> PSRANTKVIVVGGGGTIGSSTALHLVRSGYTPSNVTVLDAYPIPSSQSAGNDLNKIMDADADPAADAARQMWNEDELFKKFFHNTGRLDCAHGEKDIADLKKRYQNLRDWGLGATVEWLDSEDEILKRMPQLTRDQIKGWKAIFSKDGGWLAAAKAIKAIGEYLRDQGVRFGFYGAGSFKQPLLAEGVCIGVETVDGTRYYADKVVLAAGAWSPTLVELQEQCVSKAWVYGHIQLTPEEAARYKNSPVVYNGDVGFFFEPNEHGIIKVCDEFPGFTRFKMHQPFGAKAPKRISVPRSHAKHPTDTIPDASIVRIRRAIATFMPQFKNKPLFNQAMCWCTDTADGHLLICEHPEWKNFYLATGDSGDSFKLLPIIGKYVVELLEGTLADELAHKWRWRPGSGDALKSRREAPAKDLADMPGWNHD

Fructosyl peptide oxidases (FPOX) are deglycating enzymes that find application as key enzymatic components in diabetes monitoring devices. The inability of wild type FPOXs to act on intact proteins is the most critical issue limiting both their diabetes detection efficiency and their protein deglycation potential. This is due to their buried active site and narrow access tunnel, as determined in multiple crystal structures. In that account, using a rational design approach involving a five-amino acid deletion at the entrance of the active site and a number of further mutations, we described a stable PnFPOX mutant (named L3-35A) that, relative to the wild type enzyme, features a significantly wider and shorter access tunnel.

In the present study, we set out to enhance the thermal stability of the L3-35A mutant by implementing a methodological approach whereby different thermal stabilization strategies are tested in parallel and their efficiency compared. These various strategies involved mutations to either improve the RMSF of the protein (generating mutants hereafter referred to as D-series mutants), increase the number of salt bridges (C-series mutants) or form disulfide bonds (X-series mutants). Our MD-based ranking led to the selection of six candidate mutants (C16, D02, X01, X02A, X04, and X07) for experimental production and characterization. The D02 variant, which relative to L3-35A features two additional mutations (V110R and D115G), shows an increase in Tm of ≈ 1.5 °C with respect to the parent enzyme. We observed that the activity of the enzyme variants towards fK and fV remained similar to that of the parent enzyme, with a slight increase of activity in the case of D02 and a slight decrease in all the other cases. Overall, we observed that the activity of these mutant enzymes is several folds lower than that of PnFPOX, the naturally occurring enzyme. Also, similarly to the parent enzyme, none of these mutants shows any activity towards the dipeptide or the hexapeptide. In this process, while the amino acids that are directly involved in the catalytic function were not modified, some tunnel-lining residues were replaced. This could explain the reduced activity of both the L3-35A enzyme previously reported and its thermally-stabilized mutants described so far (D02, C16, X01, X02A, X04, X07). At the structural level, the tridimensional architecture of all mutants reported herein is maintained, confirming that our mutagenesis campaign did not impair the conformational stability of the enzyme. We then compared the residues in the catalytic site (W235, E278, G372, R415) of our mutants with those of the WT enzyme.>GSGIALSRLAQERKAWRKDHPFGFVAVPTKNPDGTMNLMNWECAIPGAAGTPWAGGLFKLRMLFKDDYPSSPPKCKFEPPLFHPNVYPSG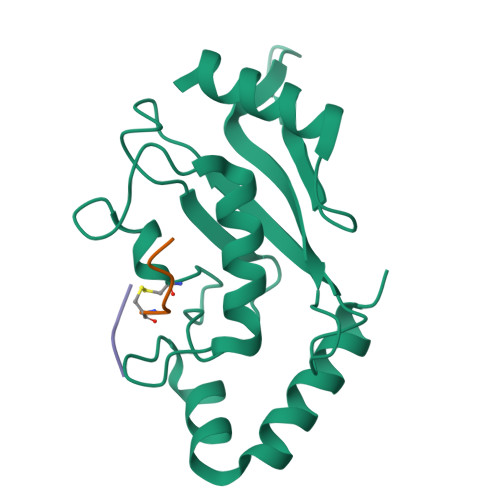TVCLSILEEDKDWRPAITIKQILLGIQELLNEPNIQDPAQAEAYTIYAQNRVEYEKRVRAQAKKFAPS[4x];>XLRLRGC[4x];>XIKQE[4x]> MFRLNSLSALAELAVGSRWYHGGSQPIQIRRRLMMVAFLGASAVTASTGLLWKRAHAESPPCV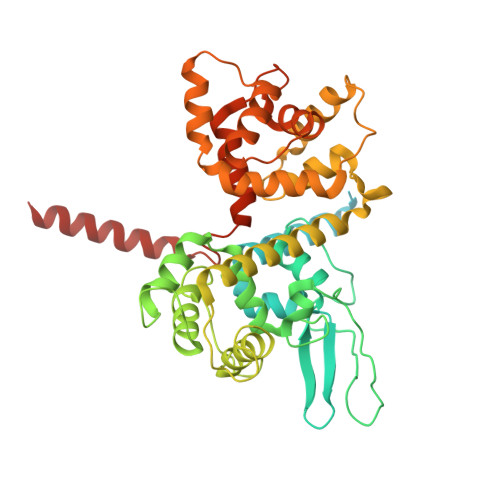DNLKSDIGDKGKNKDEGDVCNHEKKTADLAPHPEEKKKKRSGFRDRKVMEYENRIRAYSTPDKIFRYFATLKVISEPGEAEVFMTPEDFVRSITPNEKQPEHLGLDQYIIKRFDGKKISQEREKFADEGSIFYTLGECGLISFSDYIFLTTVLSTPQRNFEIAFKMFDLNGDGEVDMEEFEQVQSIIRSQTSMGMRHRDRPTTGNTLKSGLCSALTTYFFGADLKGKLTIKNFLEFQRKLQHDVLKLEFERHDPVDGRITERQFGGMLLAYSGVQSKKLTAMQRQLKKHFKEGKGLTFQEVENFFTFLKNINDVDTALSFYHMAGASLDKVTMQQVARTVAKVELSDHVCDVVFALFDCDGNGELSNKEFVSIMKQRLMRGLEKPKDMGFTRLMQAMWKCAQETAWDFALPKQ~{N}-[[3-(4-methoxyphenyl)-1,2,4-oxadiazol-5-yl]methyl]-2-(4-nitrophenyl)-~{N}-propan-2-yl-ethanamide | C21 H22 N4 O5 | 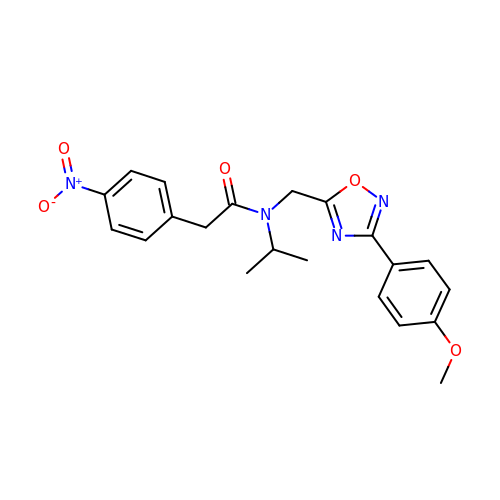QZJNXTJRNWXSBP-UHFFFAOYSA-N> MMIRVAIGGPRGKMGQEAVHTVMNNENMELVAVLDHKDIGDLLSESPNFPASYEVPVFLNLESLIVTIKPDVFLDLTTPHQVFEHTMLCLQNNVRPVIGTTGFTDEQLQQCTILAEVNKLGCIVAPNFAIGAVLMMKFASLAAAYFPDVEIIEMHHDQKLDAPSGTAYKTAQMIAEVRPSHKQGHPNEKETLEGARGASYDGIPIHSVRLPGLIAHQQILFGGEGQLFTLRHDSYNRQSFMSGVTFSINQVMEIKELVYGLENIL

DHDP reductase (DHDPR; dapB) is a branching enzyme associated with two described pathways and that reduces DHDP to tetrahydroDPA using NAD(P)H as a cofactor. DHDPR has two domains, including an N-terminal nucleotide-binding domain and a C-terminal domain for substrate binding and tetramerization. To address these issues, we determined the structure and characterized the biochemical properties of DHDPR from the psychrophilic bacterium Paenisporosarcina sp. TG-14 (PaDHDPR) isolated from sediment-laden, stratified basal ice from Taylor glacier, McMurdo dry valley, Antarctica29. The results of isothermal titration calorimetry (ITC) and enzyme activity assays demonstrated that PaDHDPR has a strong preference for NADPH as a cofactor.

DPA is a competitive inhibitor of DHDPR and has a structure similar to DHDP, a PaDHDPR substrate. The crystal structure of DPA-bound PaDHDPR was also obtained in the hexagonal space group P6422 and solved by molecular replacement using the apo form as a search model. Electron density corresponding to DPA was observed in the substrate-binding site of the C-terminal domain. Structural superposition of apo and DPA-bound PaDHDPR revealed that the two conformations were highly similar, with a root-mean-square deviation of 0.54 Å (over 244 Cα atoms). This suggests that DPA alone cannot induce domain closure of PaDHDPR. The apo and DPA-bound forms of PaDHDPR were in an open state, whereas the DPA/NADPH-bound enzyme was in a closed state. DPA binding in PaDHDPR induced a small change in the α5–β5 loop region; however, it is unlikely that the change was due to DPA binding alone, as the distance between the loop and DPA is approximately 9 Å.4-AMINO-3-HYDROXYBENZOIC 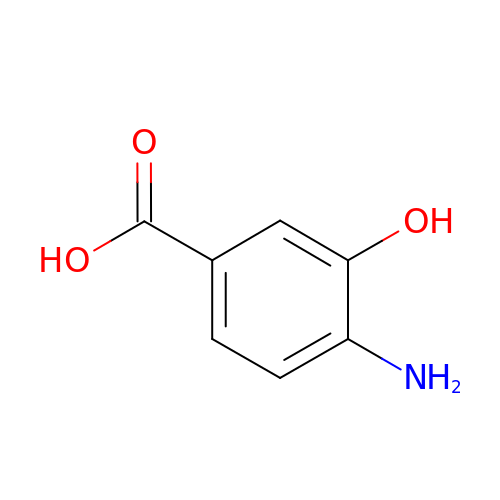ACID | C7 H7 N O3 | NFPYJDZQOKCYIE-UHFFFAOYSA-N>MGLMNAFDSQTEDSSPAIGRNLRSRPLARKKLSEMVEEELEQMIRRREFGEGEQLPSERELMAFFNVGRPSVREALAALKRKGLVQINNGERARVSRPSADTIIGELSGMAKDFLSHPGGIAHFEQLRLFFESSLVRYAAEHATDEQIDLLAKALEINSQSLDNNAAFIRSDVDFHRVLAEIPGNPIFMAIHVALLDWLIAARPTVTDQALHEHNNVSYQQHIAIVDAIRRHDPD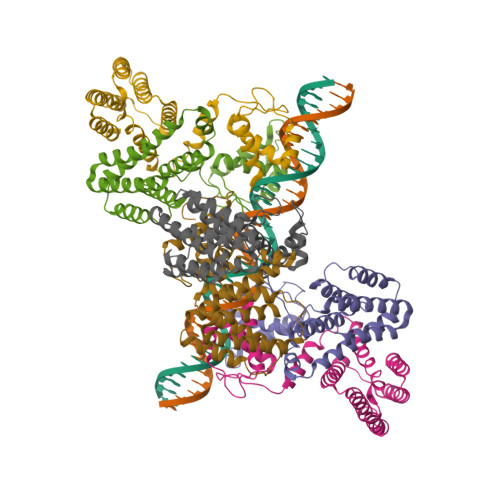EADRALQSHLNSVSATWHAFGQTTNKKK[6x]> MIKNEIKILSDIEHIKKRSGMYIGSSANEMHERFLFGKWESVQYVPGLVKLIDEIIDNSVDEGIRTKFKFANKINVTIKNNQVTVEDNGRGIPQAMVKTPTGEEIPGPVAAWTIPKAGGNFGDDKERVTGGMNGVGSSLTNIFSVMFVGETGDGQNNIVVRCSNGMENKSWETIPGKWKGTRVTFIPDFMSFETNELSQVYLDITLDRLQTLAVVYPDIQFTFNGKKVQGNFKKYARQYDEHAIVQEQENCSIAVGRSPDGFRQLTYVNNIHTKNGGHHIDCVMDDICEDLIPQIKRKFKIDVTKARVKECLTIVMFVRDMKNMRFDSQTKERLTSPFGEIRSHIQLDAKKISRAILNNEAILMPIIEAALARKLAAEKAAETKAAKKASKA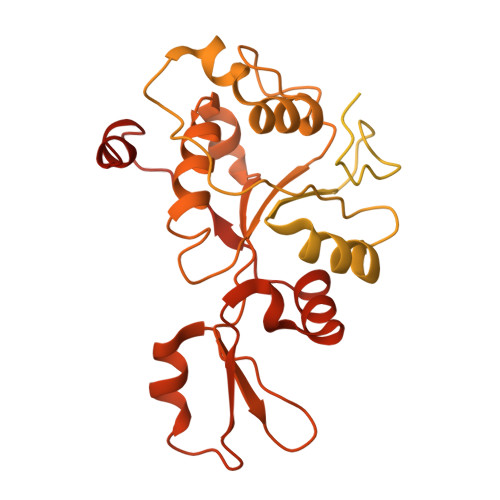KVHKHIKANLCGKDADTTLFLTEGDSAIGYLIDVRDKELHGGYPLRGKVLNSWGMSYADMLKNKELFDICAITGLVLGEKAENLNYHNIAIMTDADHDGLGSIYPSLLGFFSNWPELFEQGRIRFVKTPVIIAHVGKKQEWFYTVAEYESAKDALPKHSIRYIKGLGSLEKSEYREMIQNPVYDVVKLPENWKELFEMLMGDNADLRKEWMSQHHHHHH METHYL N-[(4-METHYLPHENYL)SULFONYL]GLYCYL-3-[AMINO(IMINO)METHYL]-D-PHENYLALANINATE | C20 H24 N4 O5 S | 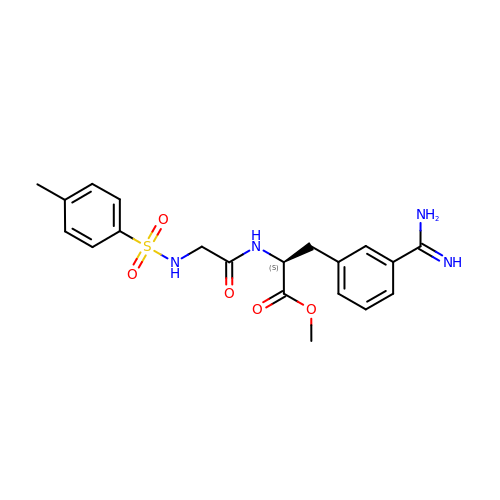YAEIKQDHLCFGAA-KRWDZBQOSA-N>[2x]AGGHGDVGMHVKEKEKNKDENKRKDEERNKTQEEHLKEIMKHIVKIEVKGEEAVKKEAAEKLLEKVPSDVLEMYKAIGGKIYIVDGDITKHISLEALSEDKKKIKDIYGKDALLHEHYVYAKEGYEPVLVIQSSEDYVENTEKALNVYYEIGKILSRDILSKINQPYQKFLDVLNTIKNASDSDGQDLLFTNQLKEHPTDFSVEFLEQNSNEVQEVFAKAFAYYIEPQHRDVLQLYAPEAFNYMDKFNEQEINLSLEELKDQRMLSRYEKWEKIKQHYQHWSDSLSEEGRGLLKKLQIPIEPKKDDIIHSLSQEEKELLKRIQIDSSDFLSTEEKEFLKKLQIDIRDSLSEEEKELLNRIQVDSSNPLSEKEKEFLKKLKLDIQPYDINQRLQDTGGLIDSPSINLDVRKQYKRDIQNIDALLHQSIGSTLYNKIYLYENMNINN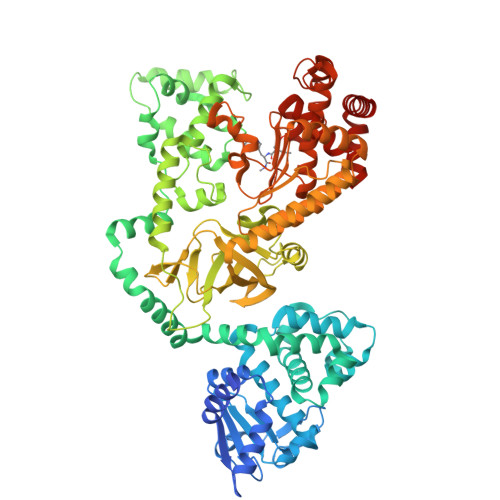LTATLGADLVDSTDNTKINRGIFNEFKKNFKYSISSNYMIVDINERPALDNERLKWRIQLSPDTRAGYLENGKLILQRNIGLEIKDVQIIKQSEKEYIRIDAKVVPKSKIDTKIQEAQLNINQEWNKALGLPKYTKLITFNVHNRYASNIVESAYLILNEWKNNIQSDLIKKVTNYLVDGNGRFVFTDITLPNIAEQYTHQDEIYEQVHSKGLYVPESRSILLHGPSKGVELRNDSEGFIHCFGHAVDDYAGYLLDKNQSDLVTNSKKFIDIFKEEGSNLTSYGRTNEAEFFAEAFRLMHSTDHAERLKVQKNAPKTFQFINDQIKFIINS>GSMGKPFFTRNPSELKGKFIHTKLRKSSRGFGFTVVGGDEPDEFLQIKSLVLDGPAALDGKMETGDVIVSVNDTCVLGHTHAQVVKIFQSIPIGASVDLELCRGYPLGSSAYGSVKAYTNFDAERDALNIETAIKTKGVDEVTIVNILTNRSNEQRQDIAFAYQRRTKKELASALKSALSGHLETVILGLLKTPAQYDASELKASMKGLGTDEDSLIEIICSRTNQELQEINRVYKEMYKTDLEKDIISDTSGDFRKLMVALAKGRRAEDGSVIDYELIDQDARDLYDAGVKRKGTDVPKWISIMTERSV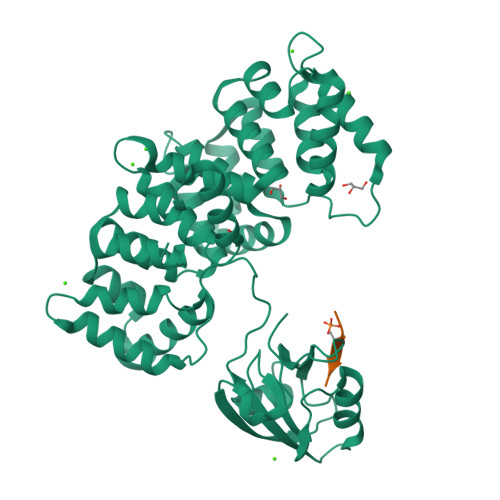PHLQKVFDRYKSYSPYDMLESIRKEVKGDLENAFLNLVQCIQNKPLYFADRLYDSMKGKGTRDKVLIRIMVSRSEVDMLKIRSEFKRKYGKSLYYYIQQDTKGDYQKALLYLCGGDD[2x];> KLPSTTL> NAESSNPPQKMAFKAFGSPKKEKKESLSDF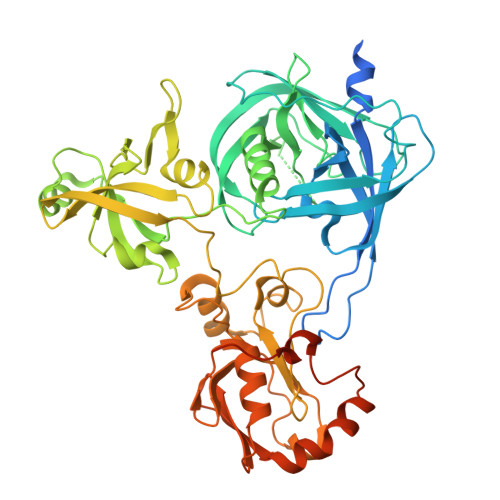SRDQQTDPAKIHDASFLNAVVKVYCTHTAPDYSLPWQKQRQFTSTGSAFMIGDGKLLTNAHCVEHDTQVKVKRRGDDRKYVAKVLVRGVDCDIALLSVESEDFWKGAEPLRLGHLPRLQDSVTVVGYPLGGDTISVTKGVVSRIEVTSYAHGSSDLLGIQIDAAINPGNSGGPAFNDQGECIGVAFQVYRSEETENIGYVIPTTVVSHFLTDYERNGKYTGYPCLGVLLQKLENPALRECLKVPTNEGVLVRRVEPTSDASKVLKEGDVIVSFDDLHVGCEGTVPFRSSERIAFRYLISQKFAGDIAEIGIIRAGEHKKVQVVLRPRVHLVPYHIDGGQPSYIIVAGLVFTPLSEPLIEEECEDTIGLKLLTKARYSVARFRGEQIVILSQVLANEVNIGYEDMNNQQVLKFNGIPIRNIHHLAHLIDMCKDKYLVFEFEDNYVAVLEREASNSASLCILKDYGIPSERSADLLEPYVDPIDDTQALDQGIGDSPVSNLEIGFDGLVWA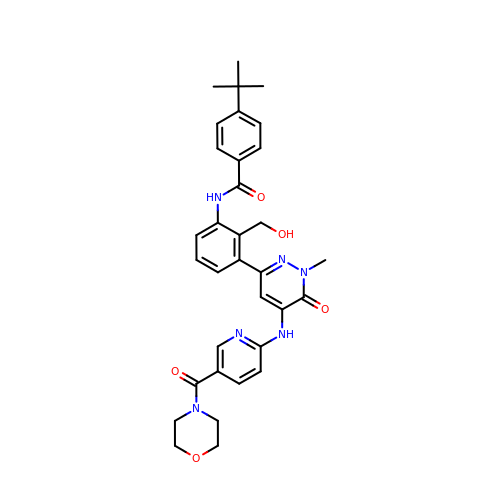4-tert-butyl-N-[2-(hydroxymethyl)-3-(1-methyl-5-{[5-(morpholine-4-carbonyl)pyridin-2-yl]amino}-6-oxo-1,6-dihydropyridazin-3-yl)phenyl]benzamide | C33 H36 N6 O5 | SXPUZMXHGHCZEG-UHFFFAOYSA-N> GKITFYEDRGFQGRHYECSSDHSNLQPYFSRCNSIRVDSGCWMLYEQPNFQGPQYFLRRGDYPDYQ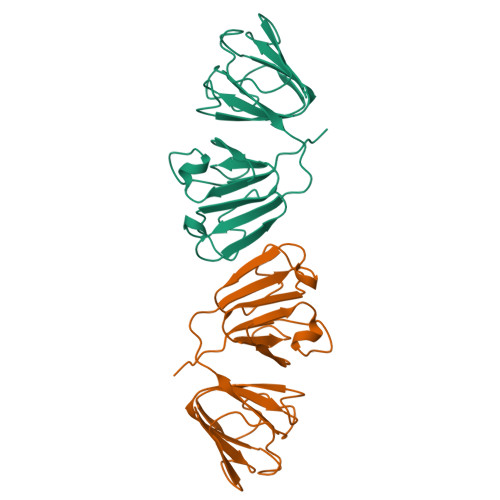QWMGLNDSIRSCRLIPHTGSHRLRIYEREDYRGQMVEITEDCSSLHDRFHFSEIHSFNVLEGWWVLYEMTNYRGRQYLLRPGDYRRYHDWGATNARVGSLRRAVDFY> AVCGSVWGQNDLAYRCRTCEHDPTCAICVPCFQNGNHKDHDYSIMYTGGGCCDCGDTTAWKREGFC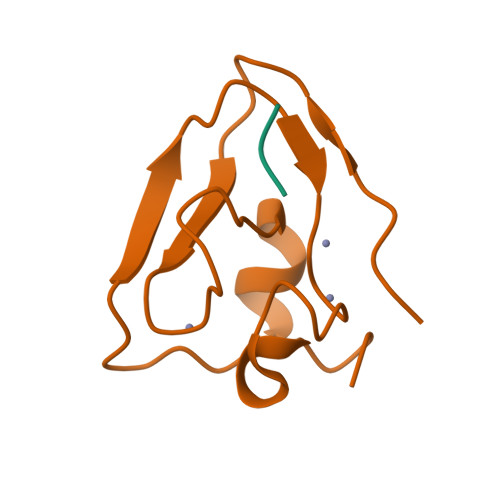SRHKGA;> RSG> GSHMEL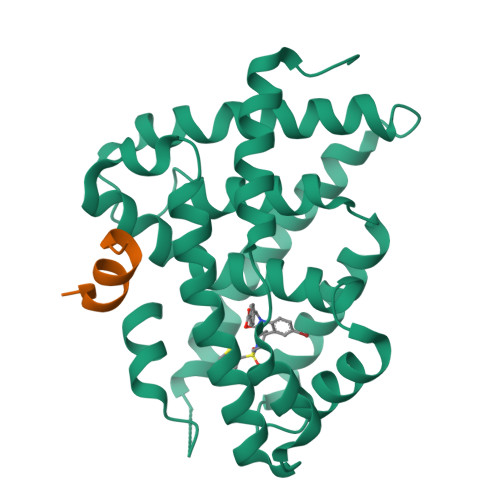TPDQQTLLHFIMDSYNKQRMPQEITNKILKEAFSAEENFLILTEMATNHVQVLVEFTKKLPGFQTLDHEDQIALLKGSAVEAMFLRSAEIFNKKLPSGHSDLLEARIRNSGISDEYITPMFSFYKSIGELKMTQEEYALLTAIVILSPDRQYIKDREAVEKLQEPLLDVLQKLCKIHQPENPQHFACLLGRLTELRTFNHHHAEMLMSWRVNDHKFTPLLCEIWDVQ;> ENALLRYLLDKD> QETLVRPKPLLLKLLKSVGAQKDTYTMKEVL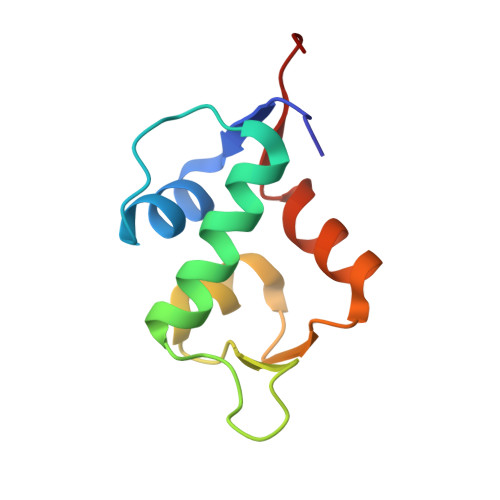FYLGQYIMTKRLYDEKQQHIVYCSNDLLGDLFGVPSFSVKEHRKIYTMIYRNLVVVNQQ>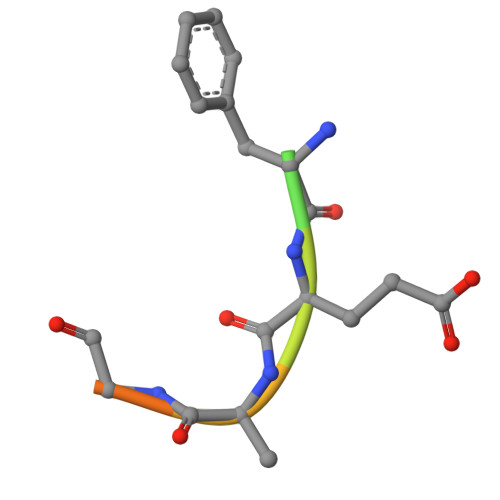 HHTFEYGDGI Enhanced ABA levels elicited in response to drought are perceived by the PYR/PYL/RCAR family of ABA receptors and the clade A subfamily of protein phosphatases type 2C (PP2Cs), which act as necessary ABA co-receptors in ternary complexes. In the resting state, PYLR/PYL/RCAR receptors display an open ABA binding cavity flanked by two highly conserved loops, named as gate/CL2/β3-β4 loop and latch/CL3/β5-β6 loop. Specifically, both gate and latch loops define a surface that enables the receptor to dock into the PP2C active site. The formation of receptor-ABA-phosphatase complexes causes the dissociation of different PP2C-SnRK2 complexes and abolishes PP2C-mediated inhibition of the SnRK2s, triggering ABA response.

We reasoned that swapping the positions of the SO2 and CH2 moieties in the SB linker might contribute to fill this cavity by promoting the formation of a hydrogen bond between the SO2 moiety of the agonist and the Lys88 side chain, increasing ligand activity. We, therefore, synthesized two new compounds incorporating the above swap, iSB07 and iSB09 (“inverted SB”). To gain insight into the structural basis of iSB agonist activity, we solved the crystal structures of CsPYL1-iSB07-HAB1, CsPYL1-iSB09-HAB1, CsPYL15m-iSB07-HAB1, and CsPYL15m-iSB09-HAB1. Consistent with our docking predictions, both iSB07 and iSB09 complexes display the hydrogen bond network to conform the Trp lock and the compounds show a hydrogen bond between the oxygen of the SO2 moiety and side-chain NH3+ of Lys88 and, unexpectedly, an additional one to the guanidinium moiety of Arg108 side chain. In addition, there are several favorable rearrangements in the conformation of the iSB07, iSB09, and SB molecules in the ternary complex with CsPYL15m compared to CsPYL1. Specifically, the structure of the sulfonamide linker displays a more likely and relaxed conformation (in terms of the torsion angles) for agonists in the ligand-binding pocket of CsPYL15m than in CsPYL1. Compared to iSB07, iSB09 contains a larger alkyl group (ethyl versus methyl) at the dihydroquinoline ring that might increase ligand activity through interaction with the 3′ tunnel for SB-01. The HAB1 IC50 values of SB, iSB07, and iSB09 combined with CsPYL15m were 876, 346, and 316 nM, respectively, which indicates that both iSB07 and iSB09 are improved versions of SB (compare Figs. 2C and 3A). The structural work provided the basis of such behavior, i.e., iSB07 and iSB09 sulfonamide linkers form additional H-bonds with respect to those observed in the SB complex. In particular, that formed between the oxygen of the SO2 moiety and the NH+ of Lys88 side-chain.

> MNNNKAEADTSSSMADPETRPTYTTHHLAIPSGVTQDEFDELKQSVVEFHTYQLSQNQCSSLLAQRIRAPNDVVWSIVRRFDQPQTYKHFIKSCSVSDNFTMAVGSTRDVNLISGLPAATSTERLDILDDDRQVLGISIIGGEHRLRNYRSVISVHGFNRDGAICTVALESYVVDVPEGNTEEDTRLFADTVVKLNLQKLVSVAESQVI;> RSVYELDCIPLWGVVSIQGNRSEMEDAFAVSPHFLKLPIKMLMGDHEGMSPSLTHLTGHFFGVYDGHGGHKVADYCRDRLHFALAEEIERIKDELCKRNTGEGRQVQWDKVFTSCFLTVDGEIEGKIGRAVVGSSDKVLEAVASETVGSTAVVALVCSSHIVVSNCGDSRAVLFRGKEAMPLSVDHKPDREDEYARIENAGGKVIQWQGARVFGVLAMSRSIGDRYLKPYVIPEPEVTFMPRSREDECLILASDGLWDVMNNQEVCEIARRRILMWHKKNGAPPLAERGKGIDPACQAAADYLSMLALQKGSKDNISIIVIDLKAQRKFKTRT>IITPALISALKTSFQKHFQDALATAPSTYLQVATVIPSTTASNTYGWLGQFPKLREWIGQRVIKDMAAQGYQITNKLFESTVGVKRTDIEDDNLGVYGPLMQEMGRAAGAHPDELVFALLKAGNANLCYDGQNFFDTDHPVYPNVDGTGTATTVSNLFAPAADPGAAWYLLDTSRSLKPLIYQERMKPSFTSMTK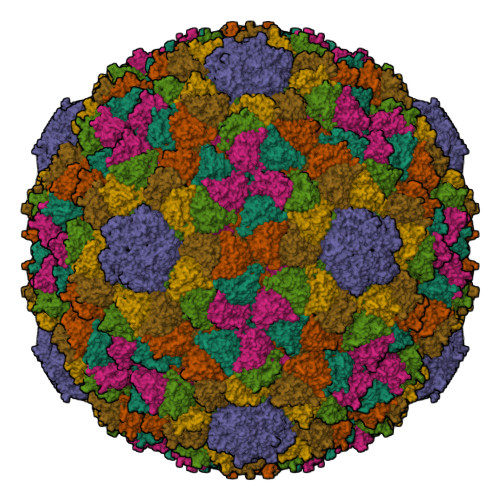EDDEQVFMADEYRYGVRSRCNVGFGFWQLAAMSTEELNQVNFEKVYDAMRNQKADGGRPLDIRPNLLVVPTTLRSKAKEVVGVQRLANGADNPNFELVQVLDTAWLN[7x]> MGANASILDGFIEDTNFSIEEIDRLRKRFMKLDKDGSGQIDKQE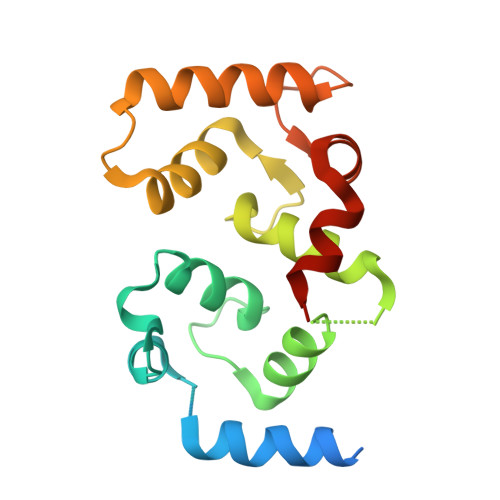FLSIPGISSNPLATRLMDVFDKDGDGSIDFEEFITGLSAFSGKSDNLNKLRFAFNIYDIDRDGYIGNGELFIVMKMMVGKNLKDEELQQIVDKTLMEADLDGDGKLNFEEFKNAVNTDTIANTLTLNMF Levansucrases (LSs) synthesize levan, a β2-6-linked fructose polymer, by successively transferring the fructosyl moiety from sucrose to a growing acceptor molecule. Recently, it was demonstrated that the LS from Bacillus subtilis (SacB) is capable of synthesizing polymer distributions with different molecular weights through two distinct elongation mechanisms. All of these structures display a single domain with a five-bladed β-propeller architecture, in which each β sheet adopts the classical “W” topology of four antiparallel β strands. In SacB, residues D86 and E342 have been identified as the nucleophile and the general acid/base, respectively, whereas D247 is the transition state stabilizer.

In this work, we present the crystal structure of an inactive double-site mutant of SacB (D86A/E342A) in complex with levan-type hexasaccharides, which are intermediate products in the synthesis of LMW levans from sucrose. The crystal asymmetric unit contains two molecules of SacB, chains A and B, each including residues 32 to 471. Each chain contains a hepta-coordinated Ca2+ ion, water molecules, and bromide ions in different sites, which are from the crystallization condition and two oligosaccharide molecules. Although the enzyme was cocrystallized with an octasaccharide, only the electronic densities of six fructose units bound by β2-6 glycosidic bonds were observable at the active site of both SacB molecules (oligosaccharide binding site 1, OB1 site). The levanhexaose molecule is oriented with its nonreducing end at the interior of the active site pocket and its reducing end protruding out of the central pocket. The levanhexaose is bound to the enzyme by 32 hydrogen bonds with the residues in the catalytic pocket, 12 to the side chains, 1 to the backbone, and the rest of the interactions with 11 residues through water molecules. In the SacB-levanhexaose structure, the oligosaccharide is used as a ligand, despite not being a donor substrate, and it is placed with its nonreducing end in an identical orientation to the fructosyl unit of sucrose and raffinose in their respective crystal structures, which allows us to define the −1, +1, +2, +3, and +4 subsites, beginning with the fructose unit inside the active site (−1) and ending with the fructose unit (+4) that extends toward the solvent. In this way, it can be established that the side chains of D117 and F182 participate in the +3 subsite, the former through a hydrogen bond with fructosyl 4 and the latter through a hydrophobic interaction. In the next subsite, the +4 subsite, residue Y237 forms CH/π stacking interactions with the fifth fructose unit of the ligand. Of interest, Y411, R360, and K363 show a different conformation in chain B, with the position of Y411 being similar to that of the apo SacB structure, while R360 and K363 shift their positions by 6.0 and 4.5 Å, respectively, away from their positions in chain A.

>[2x]KETNQKPYKETYGISHITRHDMLQIPEQQKNEKYQVPEFDSSTIKNISSAKGLDVWASWPLQNADGTVANYHGYHIVFALAGDPKNADDTSIYMFYQKVGETSIDSWKNAGRVFKDSDKFDANDSILKDQTQEWSGSATFTSDGKIRLFYTDFSGKHYGKQTLTTAQVNVSASDSSLNINGVEDYKSIFDGDGKTYQNVQQFIDEGNYSSGDNHTLRDPHYVEDKGHKYLVFEANTGTEDGYQGEESLFNKAYYGKSTSFFRQESQKLLQSDKKRTAELANGALGMIELNDDYTLKKVMKPLIASNTVTDEIARANVFKMNGKWYLFTDSRGSKMTIDGITSNDIYMLGYVSNSLTGPYKPLNKTGLVLKMDLDPNDVTFTYSHFAVPQAKGNNVVITSYMTNRGFYADKQSTFAPSFLLNIKGKKTSVVKDSILEQGQLTVNKTDPNSSSVDKLAAALEHHHHHH> MASHKLLVTPPKALLKPLSIPNQLLLGPGPSNLPPRIMAAGGLQMIGSMSKDMYQIMDEIKEGIQYVFQTRNPLTLVISGSGHCALEAALVNVLEPGDSFLVGANGIWGQRAVDIGERIGARVHPMTKDPGGHYTLQEVEEGLAQHKPVLLFLTHGESSTGVLQPLDGFGELCHRYKCLLLVDSVASLGGTPLYMDRQGIDILYSGSQKALNAPPGTSLISFSDKAKKKMYSRKTKPFSFYLDIKWLANFWGCDDQPRMYHHTIPVISLYSLRESLALIAEQGLENSWRQHREAAAYLHGRLQALGLQLFVKDPALRLPTVTTVAVPAGYDWRDIVSYVIDHFDIEIMGGLGPSTGKVLRIGLLGCNATRENVDRVTEALRAALQHCPKKKL

AGT is a hepatocyte-specific PLP dependent enzyme, belonging to the Fold Type I family, catalysing the transamination reaction between L-alanine and glyoxylate to produce glycine and pyruvate, thus leading to the removal of glyoxylate. AGT normally localises in the peroxisomes and failure of its detoxification role leads to increased levels of oxalate, coming from oxidation of glyoxylate, causing calcium oxalate precipitation in the kidney and urinary tract. Many pathogenic variants of AGT cause PH1 (primary hyperoxaluria type I), a rare autosomal recessive disorder. Our results shows that two forces generated by the salt bridge between the conserved aspartate residue and the pyridine N1 atom, and by the Schiff base linkage act as opposite springs and are responsible for the fine tilting adjustments of the pyridine plane of PLP.

Automated crystallization trials of AGT-Ma usually result in diamond shaped tetragonal crystals. We collected both crystal forms at the Elettra synchrotron in Trieste. The tetragonal crystal diffracted to 2.5 Å resolution (space group P41212; cell dimensions: a, b, c = 90.7, 90.7, 141.2), while the orthorhombic crystal yielded a high-resolution (1.7 Å) dataset.N-butyl-3-{[6-(9H-purin-6-ylamino)hexanoyl]amino}benzamide | C22 H29 N7 O2 | 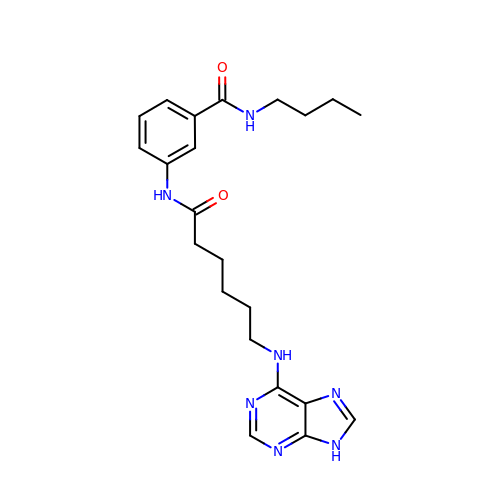WOYITRCGMUXUDE-UHFFFAOYSA-N6-[3,3-dimethyl-2-[(1~{E},3~{E},5~{E})-5-(1,3,3-trimethylindol-2-ylidene)penta-1,3-dienyl]indol-1-ium-1-yl]-~{N}-[[1-[[(1~{S},2~{R},3~{R},4~{S},6~{S})-2,3,4,6-tetrakis(oxidanyl)cyclohexyl]methyl]-1,2,3-triazol-4-yl]methyl]hexanamide 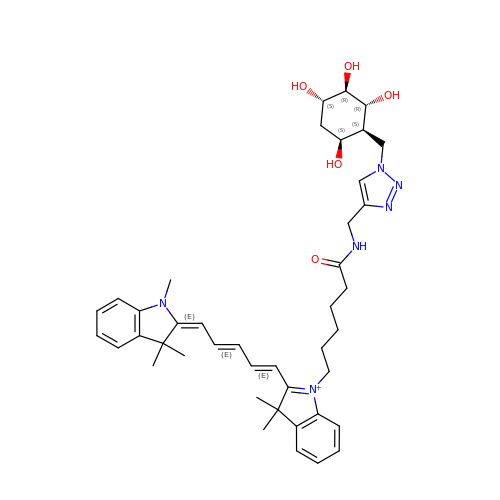| C42 H55 N6 O5 | PERJBOWNRMIYFC-ZXMFRAEJSA-O> MSALFEPYTLKDVTLRNRIAIPPMAQYMAEDGMINDWHHVHLAGLARGGAGLLVVEATAVAPEGRITPGCAGIWSDAHAQAFVPVVQAIKAAGSVPGIQIAHAGRKASANRPWEGDDHIAADDTRGWETIAPSAIAFGAHLPKVPREMTLDDIARVKQDFVDAARRARDAGFEWIELHFAHGYLGQSFFSEHSNKRTDAYGGSFDNRSRFLLETLAAVREVWPENLPLTARFGVLEYDGRDEQTLEESIELARRFKAGGLDLLSVSVGFTIPDTNIPWGPAFMGPIAERVRREAKLPVTSAWGFGTPQLAEAALQANQLDLVSVGRAHLADPHWAYFAAKELGVEKASWTLPAP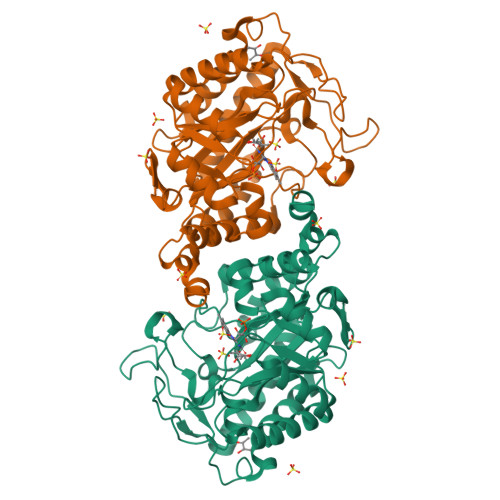YAHWLERYR>[4x]MANPEIVISSCSSHEEENRCNFNQHTSPSEELLLEDQMRRKLKFFFMNPCEKFWARGRKPWKLAIQILKIAMVTIQLVLFGLSNQMVVAFKEENTVAFKHLFLKGYIDRMDDTYAVYTQSDVYDQIIFAVNQYLQLYQVSVGNHAYENKGTDQSAMAICQHFYKRGNIYPGNDTFDIDPEIETDCFFVEPDEPFHIGTPAENKLNLTLDFHRLLTVELQFKLKAINLQTVRHQELPDCYDFTLTITFDNKAHSGRIKISLDNDISIRECKDWHVSGSIQKNTHNMMIFDAFVILTCLVSLILCIRSVISGLQLQQEFVNFFLLHYKKDVSVSDQMEFVNGWYIMIIISDILTIIGSILKMEIQAKSLTSYDVCSILLGTSTMLVWLGVIRYLGFFAKYNLLILTLQAALPNVIRFCCCAAMIYLGYCFCGWIVLGPYHNKFRSLNMVSECLFSLINGDDMFATFAKMQQKSYLVWLFSRIYLYS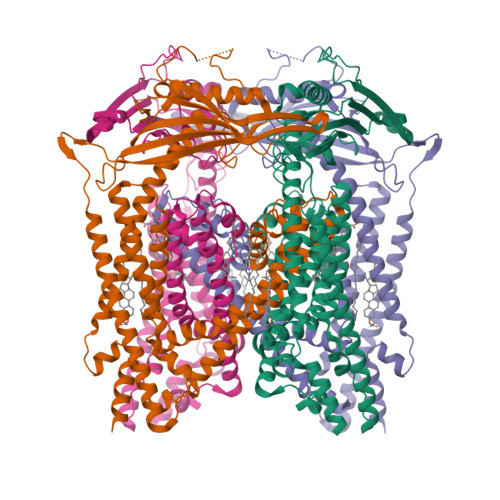FISLFIYMILSLFIALITDTYETIKHYQQDGFPETELRTFISECKDLPNSGKFRLEDDPPVSLFCCCKKSNLEVLFQ>[2x]SRKTYTLTDYLKNTYRLKLYSLRWISDHEYLYKQENNILVFNAEYGNSSVFLENSTFDEFGHSINDYSISPDGQFILLEYNYVKQWRHSYTASYDIYDLNKRQLITEERIPNNTQWVTWSPVGHKLAYVWNNDIYVKIEPNLPSYRITWTGKEDIIYNGITDWVYEEEVFSAYSALWWSPNGTFLAYAQFNDTEVPLIEYSFYSDESLQYPKTVRVPYPKAGAVNPTVKFFVVNTDSLSSVTNATSIQITAPASMLIGDHYLCDVTWATQERISLQWLRRIQNYSVMDICDYDESSGRWNCLVARQHIEMSTTGWVGRFRPSEPHFTLDGNSFYKIISNEEGYRHICYFQIDKKDCTFITKGTWEVIGIEALTSDYLYYISNEYKGMPGGRNLYKIQLSDYTKVTCLSCELNPERCQYY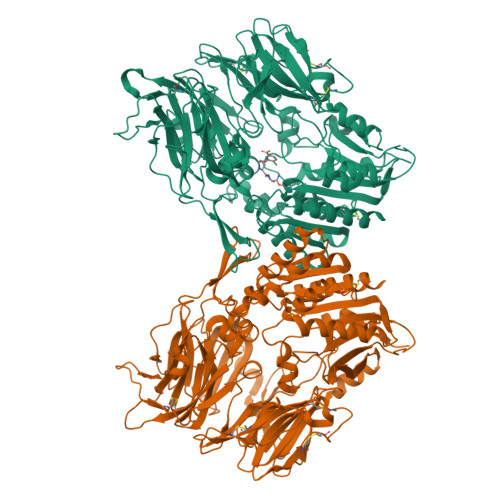SVSFSKEAKYYQLRCSGPGLPLYTLHSSVNDKGLRVLEDNSALDKMLQNVQMPSKKLDFIILNETKFWYQMILPPHFDKSKKYPLLLDVYAGPCSQKADTVFRLNWATYLASTENIIVASFDGRGSGYQGDKIMHAINRRLGTFEVEDQIEAARQFSKMGFVDNKRIAIWGWSYGGYVTSMVLGSGSGVFKCGIAVAPVSRWEYYDSVYTERYMGLPTPEDNLDHYRNSTVMSRAENFKQVEYLLIHGTADDNVHFQQSAQISKALVDVGVDFQAMWYTDEDHGIASSTAHQHIYTHMSHFIKQCFS>[8x]STTVHFEIGSIVGILITFINGPTEVYGQFLDGSPPLVWDKKDVPENKRTFKSKPRLLDIVLALYSDGCFYRAQIIDEFPSE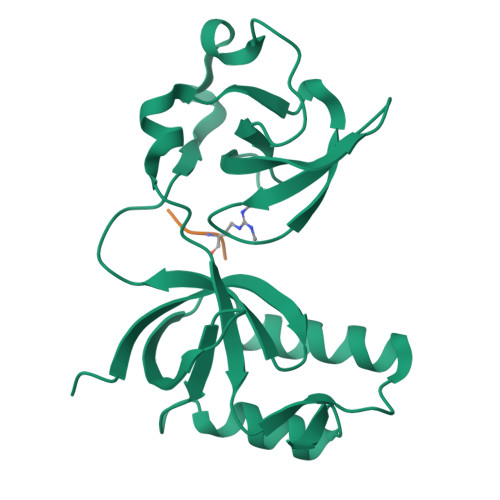YMIFYVDYGNTEFVPLSCLAPCENVDSFKPHRVFSFHIEGIVRSKNLTHQKTIECIEYLKSKLLNTEMNVHLVQRLPDGFLIRFLDDWKYIPEQLLQRNYAQVSQ;>[8x]NPVIARGRGRGRK>SNAMFKKRLIAIIGTIFIGATAMVGCNSGGSEAKSTNSVSISGSTSVGP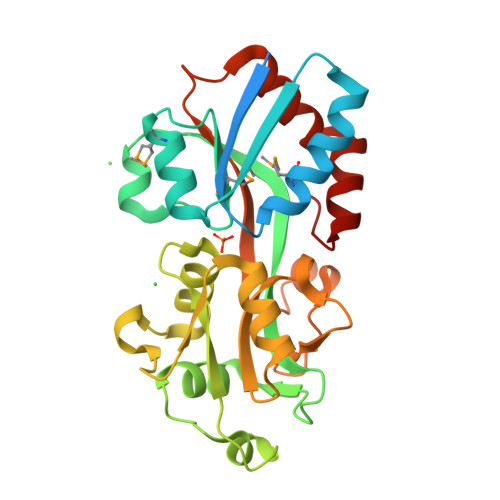VMEAEAEAFKTKKPDVSIEINQIGSSAGIKNAMEGVSEIGMASRDLKGEEKQAGLKEVEIAYDGIALITHKNNPVKDLTLVQIKDIYTGKITNWKELGGNDAPIVVVSREDGSGTRDAFQEIVGFKAEELTVNSQISDGSGNIKSLVQGNENAIGYISFSYVDDSVSAVKVDGVEATPENVLNKSYKVSRPFLAVYKEENLTESGKSFIDFILSEEGQDIVAKEHLIKVK[2x]> MSHEGEEDLLEYSDNEQEIQIDASKAAEAGETGAATSA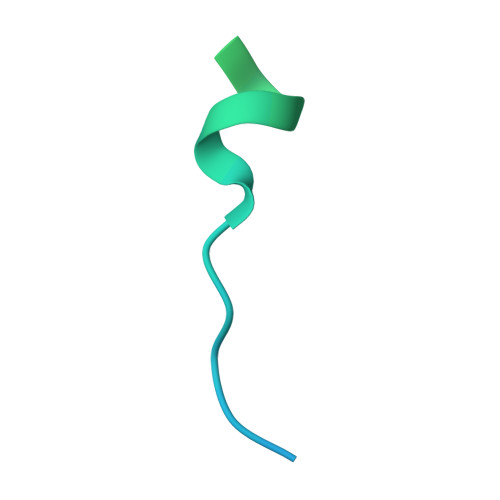TEGDNNNNTAAGDKKGS>EDENVKKFIKEFEDTKIMPVRKGTKTTRTEKFYLVFTEWVKLLQRVENNDVITTVFIKQLVEKGVISDTDNLLTFVKSSLELSVSSFKESDPTDEVFIAIDALGSLIIKLLILQDFKDDTRRDYINAIFSVIVLVFAKDHSQEGTTFNERPYFRLFSNILYEWATIRTHNFVRISDSSTRQELIEFDSVFYNTFSGYLHALQPFAFPGFSFAWVTLLSHRMLLPIMLRLPNKIGWEKLMLLIIDLFKFLDQYTSKHAVSDAVSVVYKGTLRIILGISNDMPSFLIENHYELMNNLPPTYFQLKNVILSAIPKNMTVPNPYDVDLNMEDIPACKELPEVFFDPVIDLHSLKKPVDNYLRIPSNSLLRTILSAIYKDTYDIKKGVGYDFLSVDSKLIRAIVLHVGIEAGIEYKRTSSNAVFNTKSSYYTLLFNLIQNGSIEMKYQIILSIVEQLRYPNIHTYWFSFVLMNMFKSDEWNDQKLEVQEIILRNFLKRIIVNKPHTWGVSVFFTQLINNNDINLLDLPFVQSVPEIKLILQQLVKYSKKYTTSEQDDQ[2x];>MEKFGLKALVPLLKLEDKELSSTY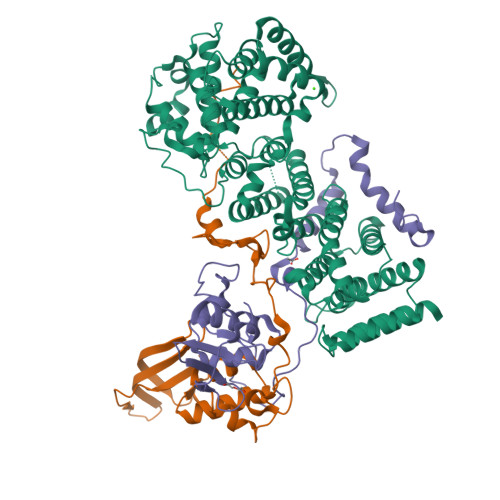DHSMTLGADLSSMLYSLGIPRDSQDHRVLDTFQSPWAETSRSEVEPRFFTPESFTNIPGVLQSTVTPPCFNSIQNDQQRVALFQDETLFFLFYKHPGTVIQELTYLELRKRNWRYHKTLKAWLTKDPMMEPIVSADGLSERGSYVFFDPQRWEKCQRDFLLFYNAIM[2x];>[2x]FDNSTLGTPTTHVSMKKKESENDSEQQLNFPPDRTDEIRKTIQHDVETNAAFQNPLFNDELKYWLDSKRYLMQPLQEMSPKMVSQLESSLLNCPDSLDADSPCLYTKPLSLPHPTSIFFPNEPIRFVYPYDVPLNLTNNENDTDNKFGKDSKAKSKKDDDIYSRTSLARIFMKFDLDTLFFIFYHYQGSYEQFLAARELFKNRNWLFNKVDRCWYYKEIEKLPPGMGKSEEESWRYFDYKKSWLARRCGNDFVYNEEDFEKL> SMCGGGSSSGDKTEITYYQFSAPADGKALDEMVKEFEKQNPDIKVNVQTIAFNDYFTKLQTQIAGGDAPDAFELNYETFMQYAEKGVLADLTSYIEKDKDFDPSTLNKQAYDAFKYDGKQYGMVESFSNVVTI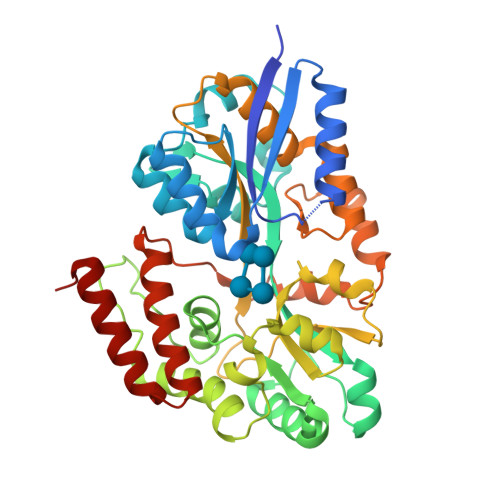YNKDLFDKAGVEYPTADWTWKDEEAAAKKLTDAKNKVWGTSQPVTMNEFYKVAAQNGGSIFNEDLTETTINSPENVEALTHLTNEVTDSKVAPSPADLSGQLPEDLFMNGQIAMLHTGIWLFDMFQDAPFKWDVQVEAGNTQKATHFFANGIGVSKDSDKKEAAFKFASFMSANEEAAKIRIDNNWELPATENKEILQPYLDATPPDNREAVFESLQYMVLPPVVKDWNKISDYTNSEFEKVLNGDSTPEKALKNSEDNINKTMGFK N-{4-[3-(6-fluoropyridin-3-yl)-4-oxo-4,5,6,7-tetrahydro-1H-pyrrolo[3,2-c]pyridin-2-yl]pyridin-2-yl}acetamide | C19 H16 F N5 O2 | 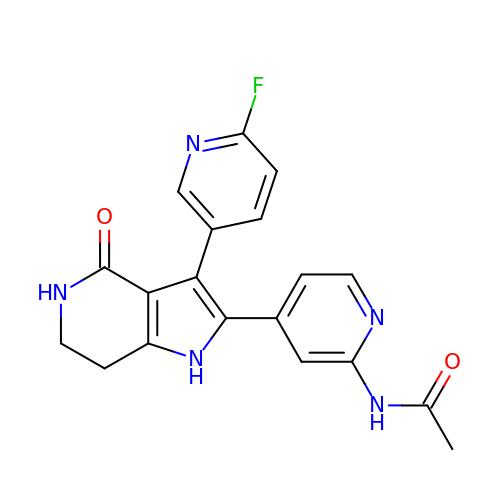TVFRIMALFOJAAL-UHFFFAOYSA-N>GSHMEKLAKNKVISIDAGRKYFTLNQLKRIVDKASELGYSDVHLLLGNDGLRFLLDDMTITANGKTYASDDVKKAIIEGTKAYYDDPNGTALTQAEVTELIEYAKSKDIGLIPAINSPGHMDAMLVAMEKLGIKNPQAHFDKVSKTTMDLKNEEAMNFVKALIGKYMDFFAGKTKIFNFGTDQYANDATSAQGWYYLKWYQLYGKFAEYANTLAAMAKERGLQPMAFNDGFYYEDKDDVQFDKDVLISYWSKGWWGYNLASPQYLASKGYKFLNTNGDWYYILGQKPEDGGGFLKKAIENTGKTPFNQLASTKYPEVDLPTVGSMLSIWADRPS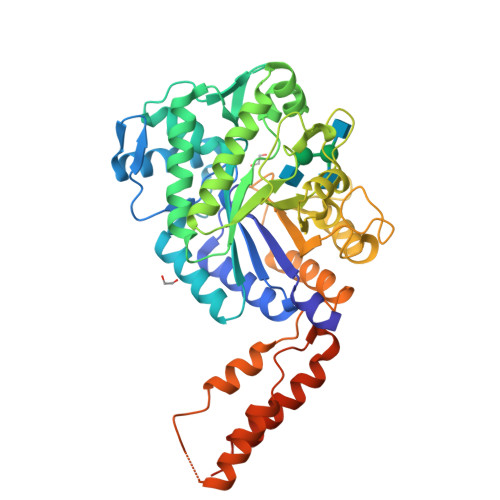AEYKEEEIFELMTAFADHNKDYFRANYNALREELAKIPTNLEGYSKESLEALDAAKTALNYNLNRNKQAELDTLVANLKAALQGLKPAVTHSGSLDENEVAANVETRP[4x]> 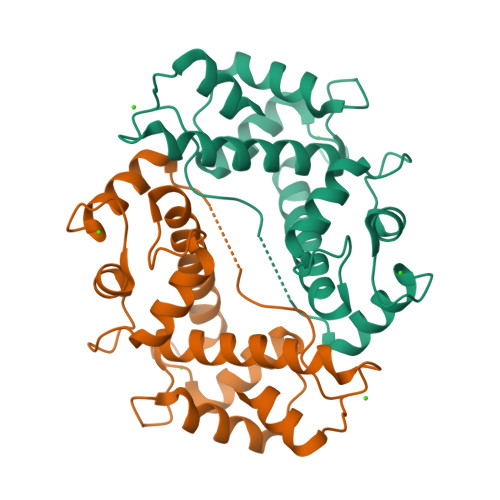MAAYSYRPGPGGGPGPAAGAALPDQSFLWNVFQRVDKDRSGVISDNELQQALSNGTWTPFNPVTVRSIISMFDRENKAGVNFSEFTGVWKYITDWQNVFRTYDRDNSGMIDKNELKQALSGFGYRLSDQFHDILIRKFDRQGRGQIAFDDFIQGCIVLQRLTDIFRRYDTDQDGWIQVSYEQYLSMVFSIV> MATDKEAKDVIDKFIDNVFNFDVLTKERIKEKDEEIKKITTDDMYEKVVYIRPYVGVIQSLNPQHVQYESFSNNGYDIEAELSFRKVSYLVDKGSIPTDSLSTLTVHLVERNQELLIDYFDEIQDVLYGEYMEEEYVFDEDVPLSTILALDLNDNLKSLSNIKYMFKGAPKENPFGTDKDVYIDTYNLLYWLYLGEDEELAYPMNINYFFTEGRFFTIFGKGHKYKVDVSKFIVGDILFFGRSDTNIGIYVGDGEFISMMGKFPKDETPIGKYKLDDYWNEFNGRVMRFDEEVYI;> MVVRFQSSMGRSLKRVDSDDLNVKGLVLATVSKINYKYQSVEVKVNNLTLGSRIGDDGSLAVPYPKSFIGRTPEGSVFGTKPLITEGSVVLIGFLNDDINSPIILSVYGDNEQNKMINTNPLDGGKFDTESVYKYSSSL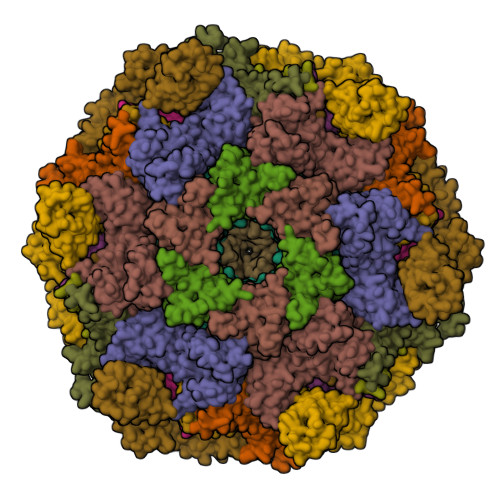YEILPSLNYKYDDGEGTSIRTYNGKSFFSMTSGEEEKPQATDFYTGTEYQDLFTSYYGNKTLIEPRIQKAPNMLFKHQGVFYDDGTPDNHITTLFISERGDIRASVLNTETQKRTTQEMSSDGSYRVIKQDDDLMLDEAQVWIEYGISEDNKFYIKNDKHKFEFTDEGIYIDDKPMLENLDESIAEAMKNLNEIQKELDDINYLLKGVGKDNLEELIESTKESIEASKKATSDVNRLTTQIAEVSGRTEGIITQFQKFRDETFKDFYEDASTVINEVNQNFPTMKTDVKTLKTKVDNLEKTEIPNIKTRLTELENNNNNADKIISDRGEHIGAMIQLEENVTVPMRKYMPIPWSKVTYNNAEFWDSNNPTRLVVPKGITKVRVAGNVLWDSNATGQRMLRILKNGTYSIGLPYTRDVAISTAPQNGTSGVIPVKEGDYFEFEAFQDSEGDRQFRADPYTWFSIEAIELETETMEKDFMLIGHRGATGYTDEHTIKGYQMALDKGADYIELDLQLTKDNKLLCMHDSTIDRTTTGTGKVGDMTLSYIQTNFTSLNGEPIPSLDDVLNHFGTKVKYYIETKRPFDANMDRELLTQLKAKGLIGIGSERFQVIIQSFARESLINIHNQFSNIPLAYLTSTFSESEMDDCLSYGFYAIAPKYTTITKELVDLAHSKGLKVHAWTVNTKEEMQSLIQMGVDGFFTNYLDEYKKI;>[4x]MKTRKLTNILSKLIDKTMAGTSKITDFTPGSASRSLLEAVSLEIEQFYILTKENIDWGIQEGIIEAFDFQKRQSKRAYGDVTIQFYQPLDMRMYIPAGTTFTSTRQEYPQQFETLVDYYAEPDSTEIVVEVYCKETGVAGNVPEGTINTIASGSSLIRSVNNEYSFNTGTKEESQEDFKRRFHSFVESRGRATNKSVRYGALQIPDVEGVYVYEETGHITVFAHDRNGNLSDTLKEDIIDALQDYRPSGIMLDVTGVEKEEVNVSATVTISNKSRIGDTLQKHIESVIRSYLNNLKTSDDLIITDLIQAIMNIDDVLIYDVSFDNLDENIIVPPQGIIRAGEIKVELK;> MRRIRRPKVRIEIVTDDNTFTLRFEDTRDYNGDEFGAKLLGFQTKNSMEDDSSVFQINMAGDTYWDKLVMANDIIRIFITPNDDPNDKEGKQERLIQVGMVSQVSKVGSYGNDQTQFRITGQSFVKPFMKFGLGVIQEVQAVLPEVGWLIDGDGDNEVKFTGSSAHEVMTGIIRRFIPYMKYNYTEKTYNTIDNYLDYDDLSSWDEFEKLTEVSAFTNFDGSLKQLMDMVTARPFNELFFKNSEKTPGKAQLVLRKTPFNPTEWRALDMIKVPTEDFIEEDVGKSDVETYSIFTATPAGMLKELNGDVFSKPQFHPELTDRYGYTKFEVENIYLSTKSGSATEDSDSSGDDNGTERGTYSKIMKDLSNYGRDNISKGIDKYTSKLSSKYKNLKKAQAKKIIEKFVKEGKVTEKEYEKITGNKVDDELTSDNRPKLTKDKLKSILKEKFKTQDDFNNSKKKKKAKTDALKELTTKYRFGNKTHATTLLDEYIKYKGEPPNDEAFDKYLKAIEGVSNVATDTGSDASDSPLVMFSRMLFNWYHGNPNFYAGDIIVLGDPKYDLGKRLFIEDKQRGDTWEFYIESVEHKFDYKQGYYTTVGVTRGLKDAILEDGKGSPHRFAGLWNQSSDFMGGLMGEDTSKELKEKGVAEKQSSGDKDGGSDSGGAQDGGSLDSLKKYNGKLPKHDPSFVQPGNRHYKYQCTWYAYNRRGQLGIPVPLWGDAADWIGGAKGAGYGVGRTPKQGACVIWQRGVQGGSPQYGHVAFVEKVLDGGKKIFISEHNYATPNGYGTRTIDMSSAIGKNAQFIYDKK;>[2x]MNNFIPQPQGLLRFLNTLDTDLTSSHMNLLDEEVSFVSKFYTPQLQLSELAKKVLTNIKTDDIPVLEREFNDNTIIHKANDTLLKVQAPRMYMILQSIVLEAYAIVNCFVENPSSLKYLTEEDVSITRENLNYVADYLGNYDDYNSVVLDLRDLDLCFSAIELQLPLIKKEANV;>[2x]MANFLKNLHPLLRRDRNKKDNQDPNFALIDALNEEMNQVEKDAIESKLQSSLKTSTSEYLDKFGDWFGVYRKTDEKDDVYRARIIKYLLLKRGTNNAIIDAIKDYLGRDDIDVSVYEPFTNIFYTNKSHLNGEDHLMGYYYRFAVINVSIGDYFPVEIIDVINEFKPAGVTLYVTYDGASTIRGGAIIKWLDGLPKIETYQEFDRFTGYDDTFYGHINMNQSKDTDNSSSDIFKTNHSLINSLDVLTGSSSVGRQYINYGYVTSYVYNPGMTSSVNQISASTEGRGQEVPTDYYMYTSTKNNNTVELSMQTTSGVSYLYNNFNFRDYMSKYRPQVDLQSDEARRIVSDYIKELSIDYYLSAVIPPDESIEIKLQVYDFSINRWLTVSINNLSFYEKNIGSNIGYIKDYLNSELNMFTRLEINAGKRDSVDIKVNYLDLMFYYYERGIYTIKPYKALIENYLDISRETYVEAFKIASLSNGDIITKTGFQPIGYLKLVGNYENTIPSTINIVAKDTDNNPIESNELDVYNTVENRNLLQSYKGVNTIAREITSTKEFTVSGWAKEIYSTNYLSKVLKPGKVYTLSFDMEITGNDPTLKSYSDNHGIYLYSNTKGIVVNGVKSMERTIGNKVSVTQTFTAPTITDHRLLIYTGRYTSDGKASTPPVFFNTVKITELKLTEGSSKLEYSPAPEDKPNVIEKGIKFNNILTNIQTLSINSDTILKNVTLYYSYYGDSWVELKTLGNISTGETTETNNLIDLYGLQTVDYSNINPMSKVSLRSIWNVKLGELNNQEGSLSNMPNDYFNAVWQDIDKLSDIELGSMRMVKDTEGGVFDGATGEIIKATLFNVGAYTDLDMLAYTLTNYTEPLTLGSSRLISELKEELLTSESFNVDNRIKVIDSIYEELPNTSIIKNGFVEREVTGSKYLDYGLYEPIEDGTRYKLIVEGEFKDNIEFISLYNSNPNFNETFIYPSEIINGVAEKEFIAKPSTEDKPRLNTDVRIYIRPYDSTISKVRRVELRKV;>[2x]MRFKKHVVQHEETMQAIAQRYYGDVSYWIDLVEHNNLKYPYLVETDEEKMKDPERLASTGDTLIIPIESDLTDVSAKEINSRDKDVLVELALGRDLNITADEKYFNEHGTSDNILAFSTNGNGDLDTVKGIDNMKQQLQARLLTPRGSLMLHPNYGSDLHNLFGLNIPEQATLIEMEVLRTLTSDNRVKSANLIDWKIQGNVYSGQFSVEIKSVEESINFVLGQDEEGIFALFE;>MPQSDGISNLHRIALRFPKEGGGYDMYRFKVNPENYTIDSPQRTTAIKTKSDIVIEDYGKDIEVINFTGTTGFRPVREADGLKTGKQKMEELQSRVSEYAMQGGSGNVSGSYLQFFNFTDDSYYKVHLAPQGLKITRSKDEPLLFRYEITLVVIGSLTEADRSAVTTEEFGNVKPNASQRVDEGIKELDKNARKTRDRNNQEISRRENTIPKSTGDNTNEGNRLKQSFPSSSIYNPRQSTNGLKGNIDNMALIIGYGDGGVSS[2x]>[6x]SLEIPSKQIDYRDVFIEFLTTFKGNNNQNKYIERINELVAYRKKSLIIEFSDVLSFNENLAYEIINNTKIILPILEGALYDHILQLDPTYQRDIEKVHVRIVGIPRVIELRKIRSTDIGKLITIDGILVKVTPVKERIYKATYKHIHPDCMQEFEWPEDEEMPEVLEMPTICPKCGKPGQFRLIPEKTKLIDWQKAVIQERPEEVPSGQLPRQLEIILEDDLVDSARPGDRVKVTGILDIKQDSPVKRGSRAVFDIYMKVSSIEVSGGSGGSSEEDEKKIKDLAKDPWIRDRIISSIAPSIYGHWELKEALALALFGGVPKVLEDTRIRGDIHILIIGDPGTAKSQMLQFISRVAPRAVYTTGKGSTAAGLTAAVVREKGTGEYYLEAGALVLADGGIAVIDEIDKMRDEDRVAIHEAMEQQTVSIAKAGIVAKLNARAAVIAAGNPKFGRYISERPVSDNINLPPTILSRFDLIFILKDQPGEQDRELANYILDVHSGKSTKNIIDIDTLRKYIAYARKYVTPKITSEAKNLITDFFVEMRKKSSETPDSPILITPRQLEALIRISEAYAKMALKAEVTREDAERAINIMRLFLESVGVDMESGKIDID

A six-subunit ATPase ring forms the central hub of the replication forks in all domains of life. This ring performs a helicase function to separate the two complementary DNA strands to be replicated and drives the replication machinery along the DNA. The helicase/ATPase rings of eukaryotes and archaea consist of six minichromosome maintenance (MCM) proteins. The MCM rings of archaeal organisms, such as Saccharolobus solfataricus, form a homohexameric ring.

To examine the mechanism of DNA translocation by the MCM hexameric helicase, we determined cryo-EM structures of a protein construct of the MCM protein from the archaeal organism Saccharolobus solfataricus (SsoMCM) in complex with the ATP analog ADP-BeF3, magnesium, and oligonucleotide. In attempting to reveal different aspects of DNA manipulation by the MCM helicase, cryo-EM structures were determined with three different oligonucleotides of different lengths and potential for secondary structure. Despite the differences of the oligonucleotides used for complex formation, each sample showed highly similar behavior with two distinct structural classes. The first class of structure is well-structured throughout and binds a very well-ordered segment of 11 nucleotides of ssDNA within the central channel at the ATPase tier. The ATPase tier is not 6-fold symmetric because the subunits form a helical “staircase” that binds encircled ssDNA. The sixth ATPase domain (red) interacts with ssDNA at the at the bottom of the staircase with just one hairpin. This subunit also loosely interacts with DNA at the top of the staircase. Specifically, transformation of class 1 with six subunits engaged to DNA to class 2 with five subunits engaged illustrates a dissociation of one subunit from DNA.>[8x]GSEQTHRAI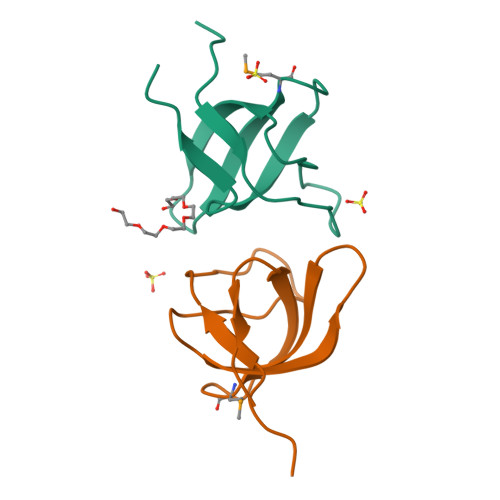FRFVPRHEDELELEVDDPLLVELQAEDYWYEAYNMRTGARGVFPAYYAIEVTK>MPPYTIVYFPVRGRCEAMRMLLADQGQSWKEEVVTIDTWMQGLLKPTCLYGQLPKFEDGDLTLYQSNAILRHLGRSLGLYGKNQREAAQMDMVNDGVEDLRGKYVTLIYTNYENGKNDYVKALPGHLKPFETLLSQNQGGKAFIVGDQISFADYNLLDLLLIHQVLAPGCLDNFPLLSAYVARLSARPKIKAFLSSPEHVNRPINGNGKQ[2x]

A large superfamily of enzymes known as glutathione transferases (GSTs; EC 2.5.1.18) catalyze the nucleophilic attack of the reduced tripeptide glutathione (GSH, L-Glu-L-Cys-Gly) on nonpolar molecules that contain an electrophilic carbon, oxygen, or sulfur atom. GSTs function as dimers consisting of two similar or different subunits, each with an average sequence length of 200–250 amino acids. Each subunit of GSTs has at least two binding sites, the G-site and the H-site, which are able to bind GSH and the electrophilic substrate, respectively. Glutathione transferases (GSTs) are involved in multidrug resistance mechanisms and play a significant part in the metabolism of alkylating anticancer drugs.

X-ray crystallography was used to determine the crystal structure of MmGSTP1-1 at 1.28 Å resolution as a complex with S-(p-nitrobenzyl)glutathione (Nb-GSH). MmGSTP1-1 was crystallized with two molecules in the asymmetric unit. A molecule of Nb-GSH was found bound in the active site of each molecule of the dimer. The amino acid residues that contribute to the binding of Nb-GSH are strictly conserved in all mammalian GSTP1-1 enzymes as well as in MmGSTP1-1. Notably, Tyr108 makes a π-π aromatic–aromatic interaction with the nitrobenzyl group of the bound Nb-GSH. An interesting finding that has not been described previously is the presence of four calcium ions in the present structure. Among them, one calcium ion was found in each of the active sites. Each of them is located in the vicinity of the H-site and forms 24 van der Waals interactions in total with protein atoms. All these interactions seem to contribute towards stabilizing and fixing the orientation of the aromatic groups of Tyr7 and Tyr108, allowing the formation of aromatic–aromatic interactions with the nitrobenzyl group of the bound Nb-GSH. Superposition of the binding site of iprodione and Nb-GSH showed that iprodione overlaps only with the nitrobenzyl group of the bound Nb-GSH.> XMNLDIHCEQLSDARWTELLPLLQQYEVVRLDDCGLTEEHCKDIGSALRANPSLTELCLRTNELGDAGVHLVLQGLQSPTCKIQKLSLQNCSLTEAGCGVLPSTLRSLPTLRELHLSDNPLGDAGLRLLCEGLLDPQCHLEKLQLEYCRLTAASCEPLASVLRATRALKELTVSNNDIGEAGARVLGQGLADSACQLETLRLENCGLTPANCKDLCGIVASQASLRELDLGSNGLGDAGIAELCPGLLSPASRLKTLWLWECDITASGCRDLCRVLQAKETLKELSLAGNKLGDEGARLLCESLLQPGCQLESLWVKSCSL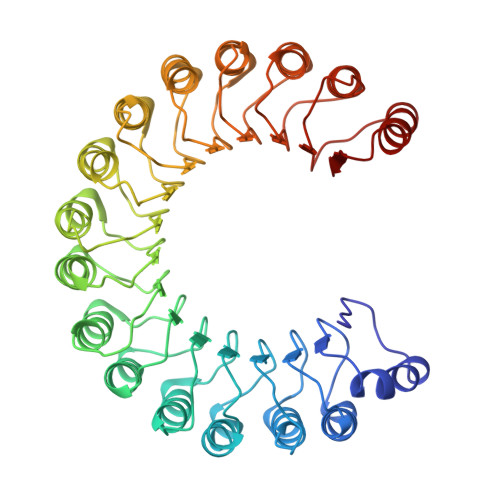TAACCQHVSLMLTQNKHLLELQLSSNKLGDSGIQELCQALSQPGTTLRVLCLGDCEVTNSGCSSLASLLLANRSLRELDLSNNCVGDPGVLQLLGSLEQPGCALEQLVLYDTYWTEEVEDRLQALEGSKPGLRVIS>MLL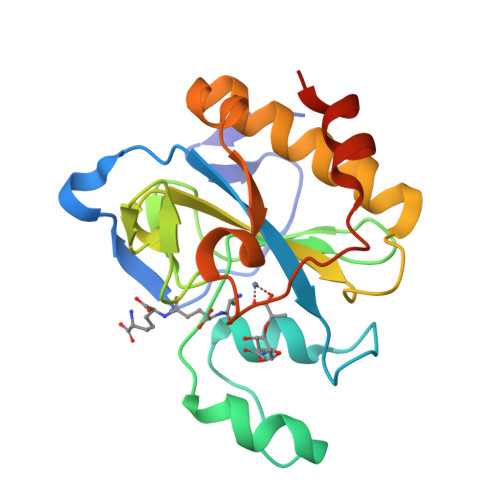DEGWLAEARRVPSPHYDCRPDDENPSLLVVHNISLPPGEFGGPWIDALFTGTIDPNAHPYFAGIAHLRVSAHCLIRRDGEIVQYVPFDKRAWHAGVSSYQGRERCNDFSIGIELEGTDTLAYTDAQYQQLAAVTNALITRYPAIANNMTGHCNIAPERKTDPGPSFDWARFRALVTPSSHKEMT[3x]>[2x]DDLYRQSLEIISRYLREQATGSKDSKPLGEAGAAGRRALETLRRVGDGVQRNHETAFQGMLRKLDIKNEDDVKSLSRVMIHVFSDGVTNWGRIVTLISFGAFVAKHLKTINQESCIEPLAESITDVLVRTKRDWLVKQRGWDGFVEFFHV

Three subsets of Bcl-2 proteins interact to determine whether cells commit to apoptosis. The BH3-only proteins then associate with anti-apoptotic Bcl-2 relatives (Mcl-1, Bcl-2, Bcl-xL, Bcl-w, Bfl-1/A1, Bcl-b) preventing their binding and inactivation of Bak and Bax (effector Bcl-2 proteins) which can then form oligomeric pores at the outer mitochondrial membrane causing cytochrome c release and caspase activation. Although the pro-survival Bcl-2 family members share several functions and structural features, the distinctive regulation of Mcl-1 makes this anti-apoptotic protein unique. Mcl-1 has attracted attention because of its established role in preventing cell death by binding and sequestering pro-apoptotic BH3 proteins, thereby mediating cancer cell survival, as well as intrinsic and acquired resistance against cytotoxic and some targeted therapies, including venetoclax.

However, during the synthesis of 3, we also isolated 4, resulting from a byproduct in the Suzuki coupling step. We then tested whether 4 could occupy more of the BH3 binding domain of Mcl-1, which should lead to improved potency. Indeed, we observed an improvement in Mcl-1 potency arising from the additional pyrazole substituent (IC50 = 0.042 µM). It is known that additional interactions could be made within the BH3-binding groove of Mcl-128–30, but it seemed that the pyrazole substituent would not extend far enough to reach the P4 pocket. A co-crystal structure of 4 in complex with Mcl-1 again revealed movement in several residue sidechains of Mcl-1 to accommodate the terminal pyrazole ring, further opening the induced-fit hydrophobic pocket, similar to what had been observed in the crystal structure of 1. Interestingly, 4 adopted a “U”-shaped conformation, with the pendant pyrazole 5-methyl group only 3.6 Å from the naphthyl 3-carbon atom. We hypothesized that constraining the molecule within a macrocycle would deliver an entropic benefit to potency, if the solution-free conformation of a macrocycle could more closely resemble the bound conformation (c.f., what appeared to be a somewhat unfavorable conformation of the linking atoms in 4). Notably, macrocycle 5 (Mcl-1 FRET IC50 = 19 nM) demonstrated improved binding affinity over its acyclic analog, 4 (Mcl-1 FRET IC50 = 42 nM).>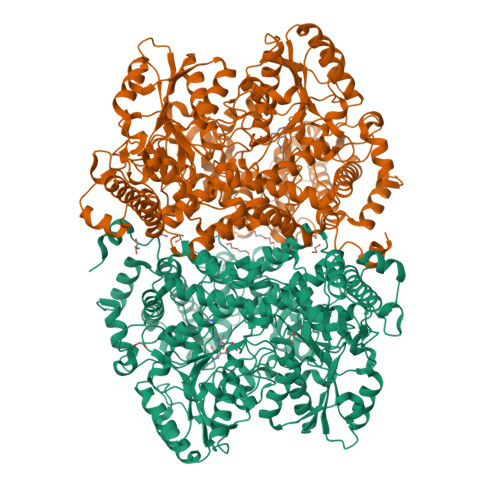[4x]MAAAGASRLLERLLPRHDDFARRHIGPGDKDQREMLQTLGLASIDELIEKTVPANIRLKRPLKMEDPVCENEILATLHAISSKNQIWRSYIGMGYYNCSVPQTILRNLLENSGWITQYTPYQPEVSQGRLESLLNYQTMVCDITGLDMANASLLDEGTAAAEALQLCYRHNKRRKFFVDPRCHPQTIAVVQTRAKYTGVLTELKLPCEMDFSGKDVSGVLFQYPDTEGKVEDFTELVERAHQSGSLACCATDLLALCILRPPGEFGVDIALGSSQRFGVPLGYGGPHAAFFAVRESLVRMMPGRMVGVTRDATGKEVYRLALQTREQHIRRDKATSNICTAQALLANMAAMFAIYHGSHGLEHIARRVHNATLILSEGLKRAGHQLQHDLFFDTLKIQCGCSVKEVLGRAAQRQINFRLFEDGTLGISLDETVNEKDLDDLLWIFGCESSAELVAESMGEECRGIPGSVFKRTSPFLTHQVFNSYHSETNIVRYMKKLENKDISLVHSMIPLGSCTMKLNSSSELAPITWKEFANIHPFVPLDQAQGYQQLFRELEKDLCELTGYDQVCFQPNSGAQGEYAGLATIRAYLNQKGEGHRTVCLIPKSAHGTNPASAHMAGMKIQPVEVDKYGNIDAVHLKAMVDKHKENLAAIMITYPSTNGVFEENISDVCDLIHQHGGQVYLDGANMNAQVGICRPGDFGSDVSHLNLHKTFCIPHGGGGPGMGPIGVKKHLAPFLPNHPVISLKRNEDACPVGTVSAAPWGSSSILPISWAYIKMMGGKGLKQATETAILNANYMAKRLETHYRILFRGARGYVGHEFILDTRPFKKSANIEAVDVAKRLQDYGFHAPTMSWPVAGTLMVEPTESEDKAELDRFCDAMISIRQEIADIEEGRIDPRVNPLKMSPHSLTCVTSSHWDRPYSREVAAFPLPFVKPENKFWPTIARIDDIYGDQHLVCTCPPMEVYESPFSEQKRASSGHHHHHH> FSDGVTAMGFQSLDTQVSIKDILRRPVLLFNHVELDPDYTGFFIPIMPPSRMMQYKSGDKETSFQRLIGRTPQAAIMNLFRFWRGSLRYTIIIHSTDGHPIYVTHVPHTGNRVYGLMKVNNLHEYTKVPIFGCGLTTEMIIPSVNPSICVEVPFDTENNWAVTFDEDAQRNYSWRDKGDTVTGHLVVTPVVSVYMSVWVEAGDDFEVSNFYGPPSVKTNDWNYAFSDEH;> GDLVIASSEPTQQFRSLTNRWMPINSIRVTVNGKRNDLLAQYYIPEDFLSTHAKCAPNTIPFETYVYGKYELEMKFVANGNKFQCGKVIISVKFDSYQADNINTGFQAALSRPHIMLDLSTNNEGVLKIPFRYHRAFVRNQTHKTATAGVRPGKFASIYVQVLSPLQTGEGGANDMFIRPFYRYTRAEFAGMSYKVPLT;> DKPKDVSSITIIPKPRLGFPHGKGKSDAVAMRVNPVALTSFQDVSAYPDEPR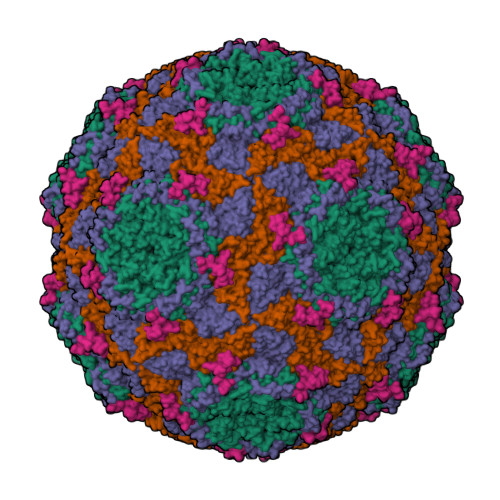TTLDIARIWGLRSTFNWGSGDEHGKELFNTVLDPGLRFYDQDYEGQITPMEYVTGLYNFWSGPIELRFDFVSNAFHTGTVIISAEYNRSSTNTDECQSHSTYTKTFHLGEQKSVHFTVPYIYDTVVRRNTASAYLPVTDYDKVDNVSRAQAMGIRAESKMRVKVRVVNVLRPVASTTSTIEVLVYMRGGKNYALHGLKQSTYWPSNSVVPIDSFPPDGYDP;> DNPHRFLPANVSNRWNEYSSAYLPRV> GFKDYGHDYHPAPKTENIKGLGDLKPGIPKTPKQNGGGKR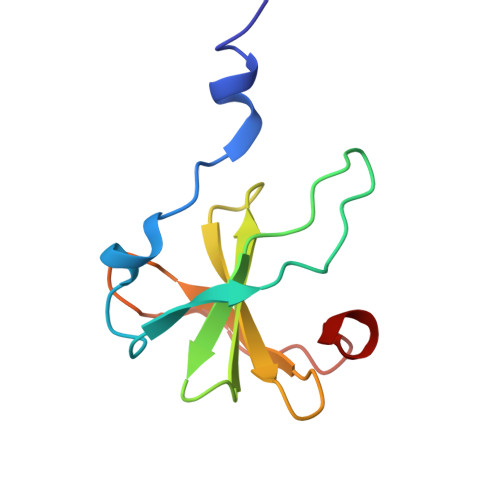KRWTGDKGRKIAEWDSQHGELEGYRASDGQHLGSFDPKTGNQLKGPDPKRNIKKYL(1) The serine protease inhibitor Kazal type 1 (SPINK1) inhibits trypsin activity in zymogen granules of pancreatic acinar cells. TRY1 adopts the typical serine protease fold containing two β-barrels sandwiching the active site cleft of the protease. The inhibitor assumes a typical Kazal domain structure with a reactive loop surrounding a central α-helix. SPINK1 binds on top of the TRY1 p.S200A active site in a substrate-like manner, creating an interface of almost 1000 Å2.

The most common variant is SPINK1 p.N34S. We solved the crystal structures of TRY1 p.S200A bound to SPINK1 WT and p.N34S at 2.9 and 2.1 Å resolution, respectively. The structures of both SPINK1 variants are mostly similar, with small differences only present in the loop orientation of the p.N34S mutation site. However, due to high flexibility of this loop, side chain conformations are poorly defined, and changes are unlikely to translate into functional effects. Asn34 or Ser34 does not directly interact with TRY1. However, the neighboring Tyr33 residue engages in a cation–pi bond with Arg101 in TRY1. This interaction causes Tyr33 to be pulled away from the core interface, making room for a sulfate ion in the SPINK1 loop. By comparing both structures, we show a slight tilt of the p.N34S variant’s α-helix. While we show minor differences between both structures, they do not translate into different binding constants or other functional differences. However, our crystal structures prove that both SPINK1 variants are mostly similar, and the minor differences we detected are unlikely to translate into functional or clinical effects.

>IVGGYNCEENSVPYQVSLNSGYHFCGGSLINEQWVVSAGHCYKSRIQVRLGEHNIEVLEGNEQFINAAKIIRHPQYDRKTLNNDIMLIKLSSRAVINARVSTISLPTAPPATGTKCLISGWGNTASSGADYPDELQCLDAPVLSQAKCEASYPGKITSNMFCVGFLEGGKDSCQGDAGGPVVCNGQLQGVVSWGDGCAQKNKPGVYTKVYNYVKWIKNTIAANS[2x];>[2x]GPGYLDSLGREAKCYSELNGCTKIYDPVCGTDGNTYPNECVLCFENRKRQTSILIQKSGPC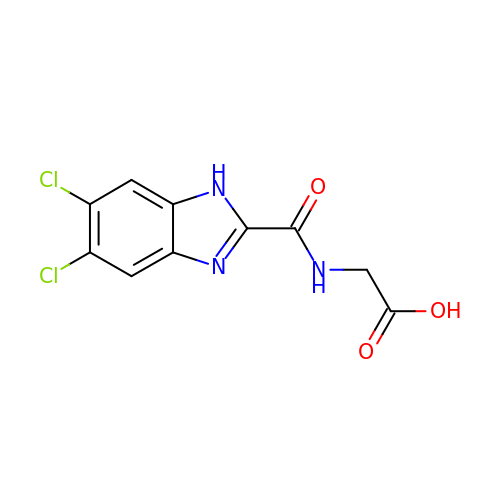N-[(5,6-dichloro-1H-benzimidazol-2-yl)carbonyl]glycine | C10 H7 Cl2 N3 O3 | ALMZPAHRESNZRJ-UHFFFAOYSA-N>GMQKLRSVKEVPQDLTNTLVNIIELRADFELAMVEQYSPWLVNAPTVDSRLFVAKLVSDELNHGWQLVRLLEEFKVKDVIERISNARLGIHKLEVSNLPLFNWEDVIAFTFLVDGAGLYQLKILKDCSFEPLS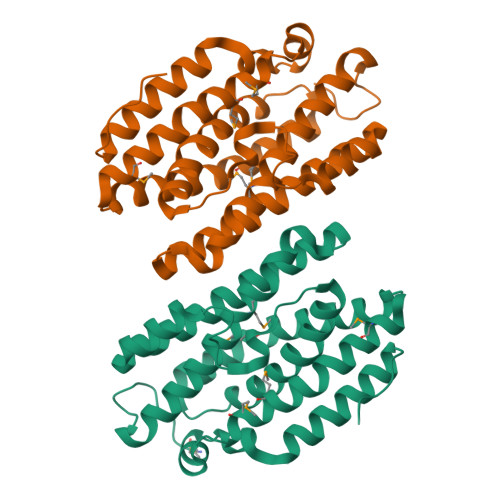TLASSMIKEEESHIFFSQNELRNYQNKNRMQGAINFWFPRAVEMLHMTWSLNETHLRDLNISDLTKNDLINGYIKTTNEELKKCGYNEVNYDKALHYNVVLK[4x]> MGSSHHHHHHSSGLVPRGSSGAFEDRDPTQFEERHLKFLQQLGKGNFGSVEMCRYDPLQDNTGEVVAVKKLQHSTEEHLRDFEREIEILKSLQHDNIVKYKGVCYSAGRRNLKLIMEYLPYGSLRDYLQKHKERIDHIKLLQYTSQICKGMEYLGTKRYIHRDLATRNILVENENRVKIGDFGLTKVLPQDKEYYKVKEPGESPIFWYAPESLTESKFSV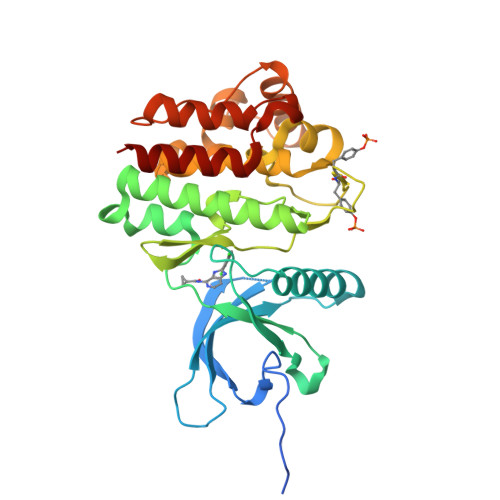ASDVWSFGVVLYELFTYIEKSKSPPAEFMRMIGNDKQGQMIVFHLIELLKNNGRLPRPDGCPDEIYMIMTECWNNNVNQRPSFRDLALRVDQIRDNMAG> MELKEIEADLERQEKEVDEDTTVTIPSAVYVAQLYHQVSKIEWDYECEPGMVKGIHHGPSVAQPIHLDSTQLSRKFISDYLWSLVDTEW;> MKQELEVLTANIQDLKEEYSRKKETISTANKANAERLKRLQKSADLYKDRLGLEIRKIYGEKLQFIFTNIDPKNPESPFMFSLHLNEARDYEVSDSAPHLEGLAEFQENVRKTNNFSAFLANVRKAFTATVYNHHHHHH;> MSVDPMTYEAQFFGFTPQTCMLRIYIAFQDYLFEVMQAVEQVILKKLDGIPDCDISPVQIRKCTEKFLCFMKGHFDNLFSKMEQLFLQLILRIPSNILLPEDKCKETPYSEEDFQHLQKEIEQLQEKYKTELCTKQALLAELEEQKIVQAKLKQTLTFFDELHNVGRDHGTSDFRESLVSLVQNSRKLQNIRDNVEKESKRLKIS;> MAEASSANLGSGCEEKRHEGSSSESVPPGTTISRVKLLDTMVDTFLQKLVAAGSYQRFTDCYKCFYQLQPAMTQQIYDKFIAQLQTSIREEISDIKEEGNLEAVLNALDKIVEEGKVRKEPAWRPSGIPEKDLHSVMAPYFLQQRDTLRRHVQKQEAENQQLADAVLAGRRQVEELQLQVQAQQQAWQALHREQRELVAVLREPE;> MTSVTRSEIIDEKGPVMSKTHDHQLESSLSPVEVFAKTSASLEMNQGVSEERIHLGSSPKKGGNCDLSHQERLQSKSLHLSPQEQSASYQDRRQSWRRASMKETNRRKSLHPIHQGITELSRSISVDLAESKRLGCLLLSSFQFSIQKLEPFLRDTKGFSLESFRAKASSLSEELKHFADGLETDGTLQKCFEDSNGKASDFSLEASVAEMKEYITKFSLERQTWDQLLLHYQQEAKEILSRGSTEAKITEVKVEPMTYLGSSQNEVLNTKPDYQKILQNQSKVFDCMELVMDELQGSVKQLQAFMDESTQCFQKVSVQLGKRSMQQLDPSPARKLLKLQLQNPPAIHGSGSGSCQHHHHHH;> GAMGGSMGKLVQSAQNEREKLQIKIDEMDKILKKIDNCLTEMETETKNLEDEEKNNPVEEWDSEMRAAEKELEQLKTEEEELQRNLLELEVQKEQTLAQIDFMQKQRNRTEELLDQLSLSEWDVVEWSDDQAVFTFVYDTIQLTITFEESVVGFPFLDKRYRKIVDVNFQSLLDEDQAPPSSLLVHKLIFQYVEEKESWKKTCTTQHQLPKMLEEFSLVVHHCRLLGEEIEYLKRWGPNYNLMNIDINNNELRLLFSSSAAFAKFEITLFLSAYYPSVPLPSTIQNHVGNTSQDDIATILSKVPLENNYLKNVVKQIYQDLFQDCHFYH;> MAGSPELVVLDPPWDKELAAGTESQALVSATPREDFRVRCTSKRAVTEMLQLCGRFVQKLGDALPEEIREPALRDAQWTFESAVQENISINGQAWQEASDNCFMDSDIKVLEDQFDEIIVDIATKRKQYPRKILECVIKTIKAKQEILKQYHPVVHPLDLKYDPDPAPHMENLKCRGETVAKEISEAMKSLPALIEQGEGFSQVLRMQPVIHLQRIHQEVFSSCHRKPDAKPENFITQIETTPTETASRKTSDMVLKRKQTKDCPQRKWYPLRPKKINLDT

Kinetochores, large layered structures built on specialized chromosome loci named centromeres, promote biorientation by binding and sensing spindle microtubules. One of the outer layer main components is a ten-subunit assembly comprising Knl1C, Mis12C and Ndc80C (KMN) subcomplexes. KMN network subunits are in turn distributed into three subcomplexes, named the Knl1 complex (Knl1C, consisting of KNL1 and ZWINT), the Mis12 complex (Mis12C, consisting of DSN1, MIS12, NSL1 and PMF1), and the Ndc80 complex (Ndc80C, consisting of NDC80HEC1, NUF2, SPC24 and SPC25). The KMN is highly elongated and docks on kinetochores and microtubules through interfaces at its opposite extremes.

We reconstituted an eight-subunit KMN network comprising the full-length Mis12C, a dimer encompassing residues 109–197 of SPC24 (SPC24109–197) and residues 92–224 of SPC25 (SPC2592–224), ZWINT and the C-terminal region of KNL1 (residues 2,021–2,342; numbering refers to isoform 1 of the CASC5 gene that encodes KNL1). The SPC24/SPC25 dimer, two tightly interacting RWD domains, caps the complex near the C-terminal tails of the Mis12C stalk, engaging in tight interactions with the C-terminal regions of DSN1 and NSL1. The RWDC of KNL1 docks against the lateral surface of the stalk, approximately 5 nm from the upper end, engaging the DSN1 and PMF1 subunits. It also captures a C-terminal motif of NSL1 that is connected to the stalk through a flexible (and largely invisible) linker. In the KMN structure, the two Mis12C heads are closely packed against each other. Comparison with a previously determined crystal structure of the complex of the Mis12C with CENP-C indicates that this closely packed (closed) conformation of the heads is incompatible with robust CENP-C binding. Specifically, the strongly positively charged DSN180–112 segment is predicted to bind at a negatively charged interface between head 1 and head 2, opposite to the CENP-C binding site.>KDRPKKPGLCPPRPQKPCVKECKNDDSCPGQQKCCNYG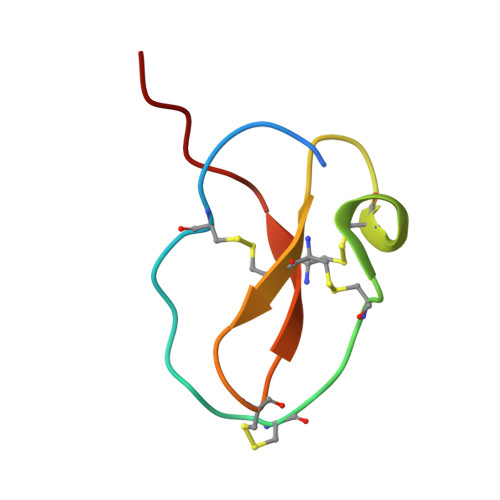CKDECRDPIFVG[2x]>[2x]CTCPNTSQRNSFLQDVPYWMLQNRSEYITQGVDSSHIVDGKKTEEIEKIATKRATIRVAQNIVHKLKEAYLSKTNRIKQKITNEMFIQMTQPIYDSLMNVDRLGI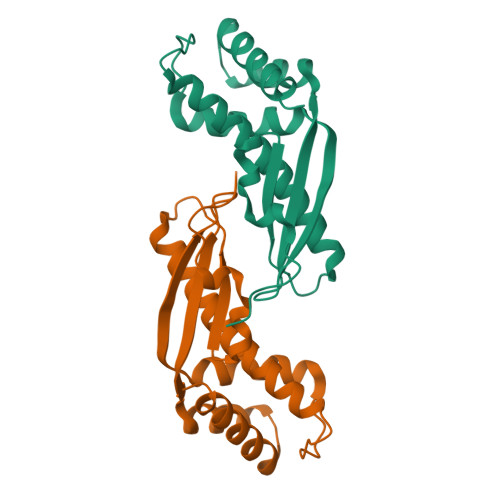YINPNNEEVFALVRARGFDKDALSEGLHKMSLDNQAVSILVAKVEEIFKDSVNYGDVKVPIAM>[4x]MGSSHHHHHHENLYFQGAESTQGQHNYKSLKYYYSKPSIELKNLDGLYRQKVTDKGVYVWKDRKDYFVGLLGKDIEKYPQG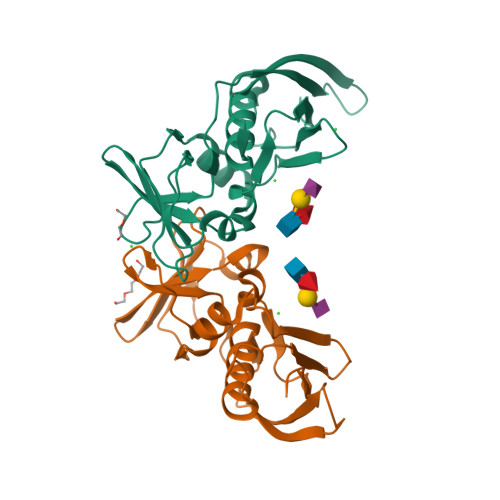EHDKQDAFLVIEEETVNGRQYSIGGLSKTNSKEFSKEVDVKVTRKIDESSEKSKDSKFKITKEEISLKELDFKLRKKLMEEEKLYGAVNNRKGKIVVKMEDDKFYTFELTKKLQPHRMGDTIDGTKIKEINVELEYK>[3x]MAQFDTEYQRLEASYSDSPPGEEDLLVHVAEGSKSPWHHIENLDLFFSRVYNLHQKNGFTCMLIGEIFELMQFLFVVAFTTFLVSCVDYDILFANKMVNHSLHPTEPVKVTLPDAFLPAQVCSARIQENGSLITILVIAGVFWIHRLIKFIYNICCYWEIHSFYLHALRIPMSALPYCTWQEVQARIVQTQKEHQICIHKRELTELDIYHRILRFQNYMVALVNKSLLPLRFRLPGLGEAVFFTRGLKYNFELILFWGPGSLFLNEWSLKAEYKRGGQRLELAQRLSNRILWIGIANFLLCPLILIWQILYAFFSYAEVLKREPGALGARCWSLYGRCYLRHFNELEHELQSRLNRGYKPASKYMNCFLSPLLTLLAKNGAFFAGSILAVLIALTIYDEDVLAVEHVLTTVTLLGVTVTVCRSFIPD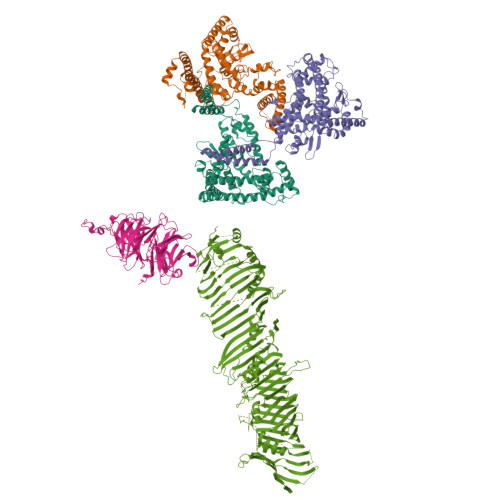QHMVFCPEQLLRVILAHIHYMPDHWQGNAHRSQTRDEFAQLFQYKAVFILEELLSPIVTPLILIFCLRPRALEIIDFFRNFTVEVVGVGDTCSFAQMDVRQHGHPQWLSAGQTEASVYQQAEDGKTELSLMHFAITNPGWQPPRESTAFLGFLKEQVQRDGAAASLAQGGLLPENALFTSIQSLQSESEPLSLIANVVAGSSCRGPPLPRDLQGSRHRAEVASALRSFSPLQPGQAPTGRAHSTMTGSGVDARTASSGSSVWEGQLQSLVLSEYASTEMSLHALYMHQLHKQQAQAEPERHVWHRRESDESGESAPDEGGEGARAPQSIPRSASYPCAAPRPGAPETTALHGGFQRRYGGITDPGTVPRVPSHFSRLPLGGWAEDGQSASRHPEPVPEEGSEDELPPQVHKV;> MTQQPLRGVTSLRFNQDQSCFCCAMETGVRIYNVEPLMEKGHLDHEQVGSMGLVEMLHRSNLLALVGGGSSPKFSEISVLIWDDAREGKDSKEKLVLEFTFTKPVLSVRMRHDKIVIVLKNRIYVYSFPDNPRKLFEFDTRDNPKGLCDLCPSLEKQLLVFPGHKCGSLQLVDLASTKPGTSSAPFTINAHQSDIACVSLNQPGTVVASASQKGTLIRLFDTQSKEKLVELRRGTDPATLYCINFSHDSSFLCASSDKGTVHIFALKDTRLNRRSALARVGKVGPMIGQYVDSQWSLASFTVPAESACICAFGRNTSKNVNSVIAICVDGTFHKYVFTPDGNCNREAFDVYLDICDDDDF;> MSRWLWPWSNCVKERVCRYLLHHYLGHFFQEHLSLDQLSLDLYKGSVALRDIHLEIWSVNEVLESMESPLELVEGFVGSIEVAVPWAALLTDHCTVRVSGLQLTLQPRRGPAPGAADSQSWASCMTTSLQLAQECLRDGLPEPSEPPQPLEGLEMFAQTIETVLRRIKVTFLDTVVRVEHSPGDGERGVAVEVRVQRLEYCDEAVRDPSQAPPVDVHQPPAFLHKLLQLAGVRLHYEELPAQEEPPEPPLQIGSCSGYMELMVKLKQNEAFPGPKLEVAGQLGSLHLLLTPRQLQQLQELLSAVSLTDHEGLADKLNKSRPLGAEDLWLIEQDLNQQLQAGAVAEPLSPDPLTNPLLNLDNTDLFFSMAGLTSSVASALSELSLSDVDLASSVRSDMASRRLSAQAHPAGKMAPNPLLDTMRPDSLLKMTLGGVTLTLLQTSAPSSGPPDLATHFFTEFDATKDGPFGSRDFHHLRPRFQRACPCSHVRLTGTAVQLSWELRTGSRGRRTTSMEVHFGQLEVLECLWPRGTSEPEYTEILTFPGTLGSQASARPCAHLRHTQILRRVPKSRPRRSVACHCHSELALDLANFQADVELGALDRLAALLRLATVPAEPPAGLLTEPLPAMEQQTVFRLSAPRATLRLRFPIADLRPEPDPWAGQAVRAEQLRLELSEPQFRSELSSGPGPPVPTHLELTCSDLHGIYEDGGKPPVPCLRVSKALDPKSTGRKYFLPQVVVTVNPQSSSTQWEVAPEKGEELELSVESPCELREPEPSPFSSKRTMYETEEMVIPGDPEEMRTFQSRTLALSRCSLEVILPSVHIFLPSKEVYESIYNRINNDLLMWEPADLLPTPDPAAQPSGFPGPSGFWHDSFKMCKSAFKLANCFDLTPDSDSDDEDAHFFSVGASGGPQAAAPEAPSLHLQSTFSTLVTVLKGRITALCETKDEGGKRLEAVHGELVLDMEHGTLFSVSQYCGQPGLGYFCLEAEKATLYHRAAVDDYPLPSHLDLPSFAPPAQLAPTIYPSEEGVTERGASGRKGQGRGPHMLSTAVRIHLDPHKNVKEFLVTLRLHKATLRHYMALPEQSWHSQLLEFLDVLDDPVLGYLPPTVITILHTHLFSCSVDYRPLYLPVRVLITAETFTLSSNIIMDTSTFLLRFILDDSALYLSDKCEVETLDLRRDYVCVLDVDLLELVIKTWKGSTEGKLSQPLFELRCSNNVVHVHSCADSCALLVNLLQYVMSTGDLHPPPRPPSPTEIAGQKLSESPASLPSCPPVETALINQRDLADALLDTERSLRELAQPSGGHLPQASPISVYLFPGERSGAPPPSPPVGGPAGSLGSCSEEKEDEREEEGDGDTLDSDEFCILDAPGLGIPPRDGEPVVTQLHPGPIVVRDGYFSRPIGSTDLLRAPAHFPVPSTRVVLREVSLVWHLYGGRDFGPHPGHRARTGLSGPRSSPSRCSGPNRPQNSWRTQGGSGRQHHVLMEIQLSKVSFQHEVYPAEPATGPAAPSQELEERPLSRQVFIVQELEVRDRLASSQINKFLYLHTSERMPRRAHSNMLTIKALHVAPTTNLGGPECCLRVSLMPLRLNVDQDALFFLKDFFTSLVAGINPVVPGETSAEARPETRAQPSSPLEGQAEGVETTGSQEAPGGGHSPSPPDQQPIYFREFRFTSEVPIWLDYHGKHVTMDQVGTFAGLLIGLAQLNCSELKLKRLCCRHGLLGVDKVLGYALNEWLQDIRKNQLPGLLGGVGPMHSVVQLFQGFRDLLWLPIEQYRKDGRLMRGLQRGAASFGSSTASAALELSNRLVQAIQATAETVYDILSPAAPVSRSLQDKRSARRLRRGQQPADLREGVAKAYDTVREGILDTAQTICDVASRGHEQKGLTGAVGGVIRQLPPTVVKPLILATEATSSLLGGMRNQIVPDAHKDHALKWRSDSAQD>[2x]MEESKVSMMNCNNEGRWSLKGTTALVTGGSKGIGYAIVEELAGLGARVYTCSRNEKELDECLEIWREKGLNVEGSVCDLLSRTERDKLMQTVAHVFDGKLNILVNNAGVVIHKEAKDFTEKDYNIIMGTNFEAAYHLSQIAYPLLKASQNGNVIFLSSIAGFSALPSVSLYSASKGAINQMTKSLACEWAKDNIRVNSVAPGVI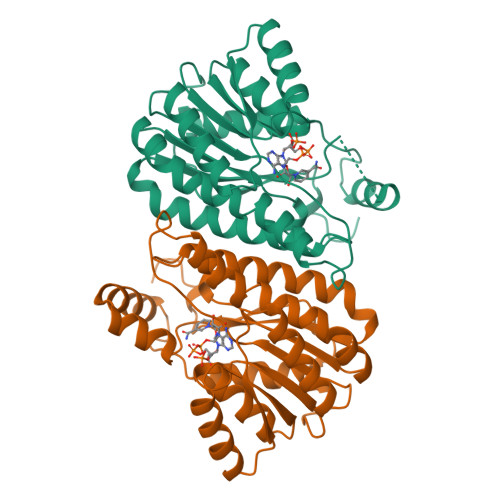LTPLVETAIKKNPHQKEEIDNFIVKTPMGRAGKPQEVSALIAFLCFPAASYITGQIIWADGGFTANGGF>[2x]GAMNAQAEEFKKYLETNGI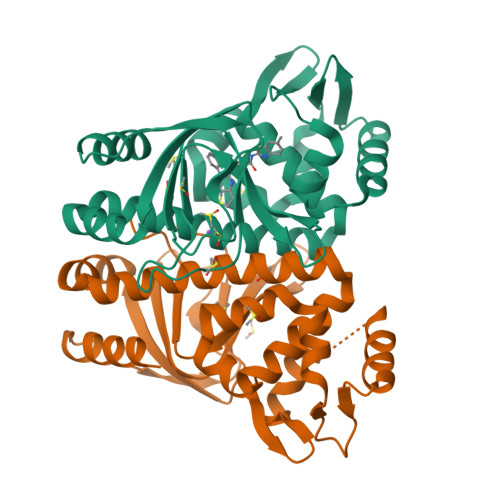KPKQFHKKELIFNQWDPQEYCIFLYDGITKLTSISENGTIMNLQYYKGAFVIMSGFIDTETSVGYYNLEVISEQATAYVIKINELKELLSKNLTHFFYVFQTLQKQVSYSLAKFNDFSINGKLGSICGQLLILTYVYGKETPDGIKITLDNLTMQELGYSSGIAHSSAVSRIISKLKQEKVIVYKNSCFYVQNLDYLKRYAPKLDEWFYLACPATWGKLN> AYVEIIEQPKQRGMRFRYKCEGRSAGSIPGERSTDTTKTHPTIKINGYTGPGTVRISLVTKDPPHRPHPHELVGKDCRDGYYEADLCPDRSIHSFQNLGIQCVKKRDLEQAISQRIQTNNNPFHVPIEEQRGDYDLNAVRLCFQVTVRDPAGRPLLLTPVLSHPIFDNRAPNTAELKICRVNRNSGSCLGGDEIFLLCDKVQKEDIEVYFTGPGWEARGSFSQADVHRQVAIVFRTPPYADPSLQAPVRVSMQLRRPSDRELSEPMEFQYLPD;> GPYLQILEQPKQRGFRFRYVC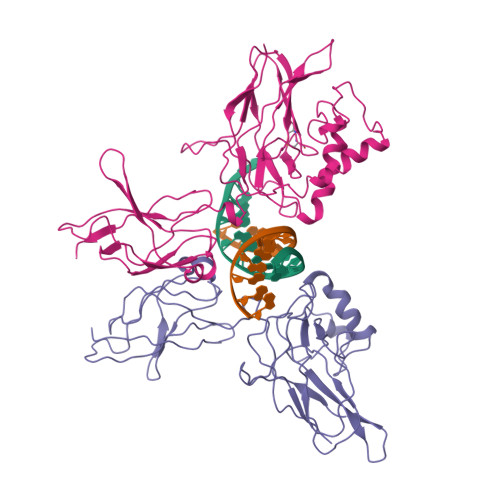EGPSHGGLPGASSEKNKKSYPQVKICNYVGPAKVIVQLVTNGKNIHLHAHSLVGKHCEDGVCTVTAGPKDMVVGFANLGILHVTKKKVFETLEARMTEACIRGYNPGLLVHSDLAYLQAEGGGDRQLTDREKEIIRQAAVQQTKEMDLSVVRLMFTAFLPDSTGSFTRRLEPVVSDAIYDSKAPNASNLKIVRMDRTAGCVTGGEEIYLLCDKVQKDDIQIRFYEEEENGGVWEGFGDFSPTDVHRQFAIVFKTPKYKDVNITKPASVFVQLRRKSDLETSEPKPFLYYPE[5-(2,4-dimethyl-1,3-thiazol-5-yl)-1H-pyrazol-3-yl]methanamine | C9 H12 N4 S | 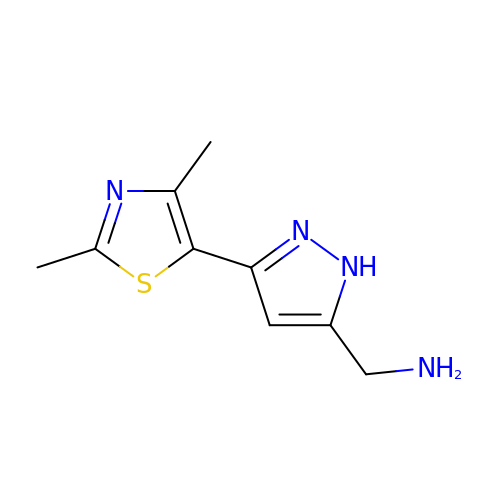IPDYKGULJOZYNW-UHFFFAOYSA-N4-NITROPHENYL 6-THIO-6-S-ALPHA-D-XYLOPYRANOSYL-BETA-D-GLUCOPYRANOSIDE | C17 H23 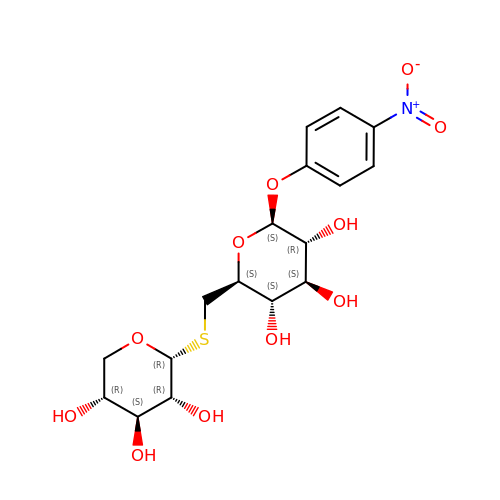N O11 S | HQYVHBCTLFPWRQ-ZMFOIVQCSA-N> MTRVRQALVALCALSLTFVTVSASASADPRETVSADAAETGSATESRPGILGTWYNQLGSVMVVTRAANGGFVGTYESAVGNAEKRYVMTGRYDSAPADGTGTAVGWTVAYRNAHRNAHSVATWSGQYVGGSQERIVTQWLLSYGTTPADQWKSTFLGHDEFTRVKPSAADVEKARQL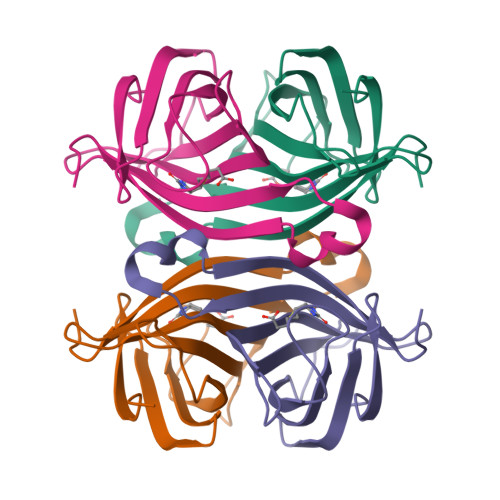GVTSANPPASDGE> VVGGTEAQRNSWPSQISLQYRSGSSWAHTCGGTLIRQNWVMTAAHCVDRELTFRVVVGEHNLNQNDGTEQYVGVQKIVVHPYWNTDDVAAGYDIA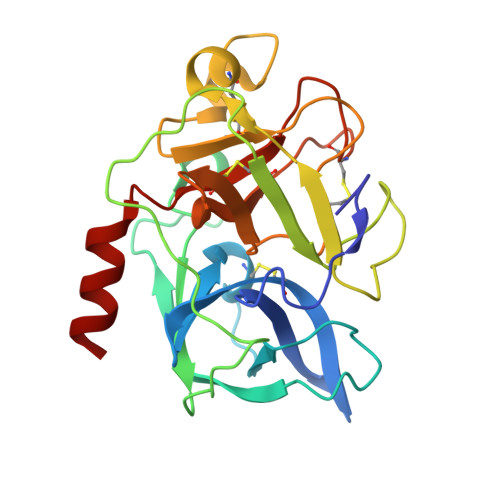LLRLAQSVTLNSYVQLGVLPRAGTILANNSPCYITGWGLTRTNGQLAQTLQQAYLPTVDYAICSSSSYWGSTVKNSMVCAGGDGVRSGCQGDSGGPLHCLVNGQYAVHGVTSFVSRLGCNVTRKPTVFTRVSAYISWINNVIASN3-naphthalen-2-ylbenzoic 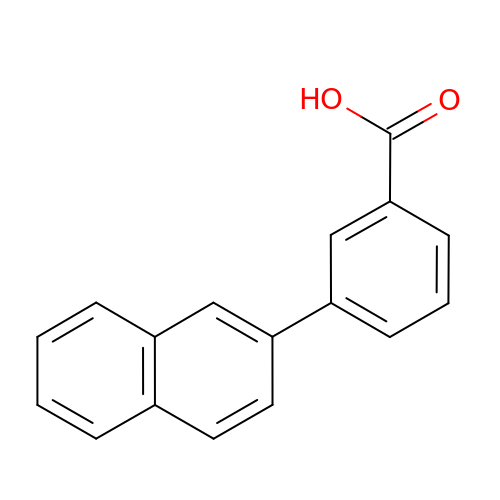acid | C17 H12 O2 | QOPDOKREBSOVNG-UHFFFAOYSA-N3-(1-methyl-2-oxo-2,3-dihydro-1H-imidazo[4,5-b]pyridin-6-yl)benzamide 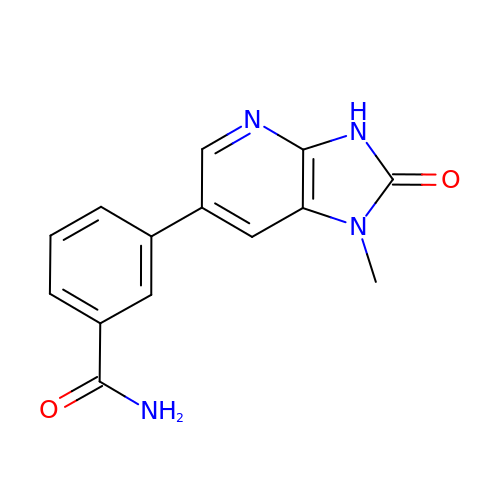| C14 H12 N4 O2 | ROERWVFKCQTDPS-UHFFFAOYSA-N> MGGSHHHHHHGMASLAPGSSRVELFKRQSSKVPFEKDGKVTERVVHSFRLPALVNVDGVMVAIADARYETSFANSLIDTVAKYSVD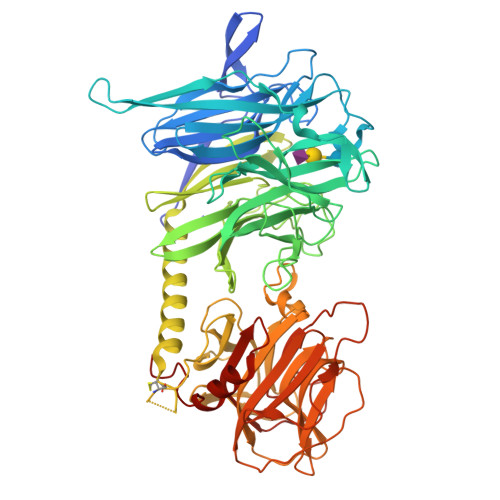DGETWETQIAIKNSRASSVSRVVDPTVIVKGNKLYVLVGSYNSSRSYWTSHGDARDWDILLAVGEVTKSTAGGKITASIKWGSPVSLKEFFPAEMEGMHTNQFLGGAGVAIVASNGNLVYPVQVTNKKKQVFSKIFYSEDEGKTWKFGKGRSAFGCSEPVALEWEGKLIINTRVDYRRRLVYESSDMGNTWLEAVGTLSRVWGPSPKSNQPGSQSSFTAVTIEGMRVMLFTHPLNFKGRWLRDRLNLWLTDNQRIYNVGQVSIGDENSAYSSVLYKDDKLYCLHEINSNEVYSLVFARLVGELRIIKSVLQSWKNWDSHLSSICTPADPAASSSERGCGPAVTTVGLVGFLSHSATKTEWEDAYRCVNASTANAERVPNGLKFAGVGGGALWPVSQQGQNQRYHFANHAFTLVASVTIHEVPKGASPLLGASLDSSGGKKLLGLSYDKRHQWQPIYGSTPVTPTGSWEMGKRYHVVLTMANKIGSVYIDGEPLEGSGQTVVPDERTPDISHFYVGGYKRSGMPTDSRVTVNNVLLYNRQLNAEEIRTLFLSQDLIGTEAHMD>LSGNSPHELKNAAQRAADWLVERQRPNGALPSRTAVIESCYKGMWALHTAGHTQAASAVADYVTSLLQPDGDIPQPREERYFLDVHYLYANGYLTIGAHVLGRFGLSRKLMSFVETMRNPATGGFRSHGPAIPGDGRCDSVSTSISGLAALYTGRVDTARSAADFLGSLWVGQPDRKNVFHAVADASGAVLTS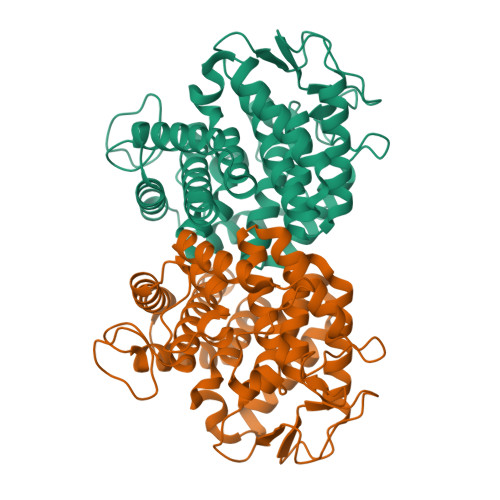DDAVAVQVRKAEGDWYFIGLPAFFLTALYEATEDRAYLDLATDLMTYMDEDCDEDAFVDSSCGKAGVAAALLYRLTGRPRYREIAEGIGTLLCERQSPYGYWSEEETGDVADLFWGDLDMTAEYVLWLDLIGRNLASGERVWAGKR[2x]>[4x]ADTIVAVELDTYPNTDIGDPNYPHIGIDIKSVRSKKTAKWNMQNGKVGTA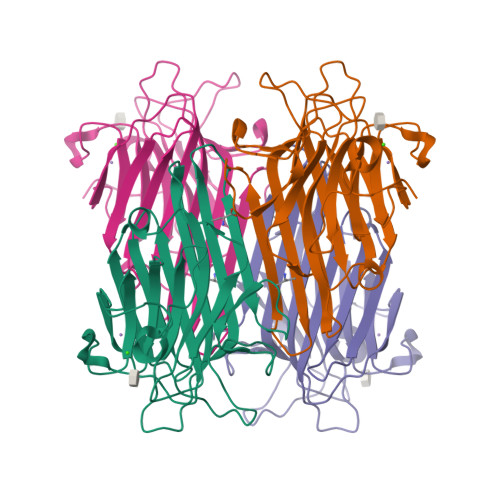HIIYNSVGKRLSAVVSYPNGDSATVSYDVDLDNVLPEWVRVGLSASTGLYKETNTILSWSFTSKLKSNSTHETNALHFMFNQFSKDQKDLILQGDATTGTDGNLELTRVSSNGSPQGSSVGRALFYAPVHIWESSAVVASFDATFTFLIKSPDSHPADGIAFFISNIDSSIPSGSTGRLLGLFPDAN>[2x]MQATKIIDGFHLVGAIDWNSR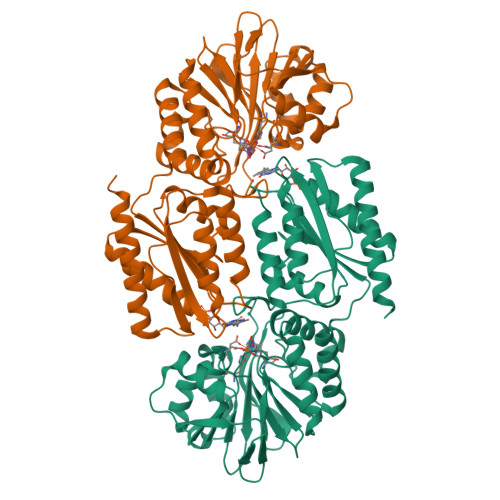DFHGYTLSPMGTTYNAYLVEDEKTTLFDTVKAEYKGELLCGIASVIDPKKIDYLVIQHLELDHAGALPALIEACQPEKIFTSSLGQKAMESHFHYKDWPVQVVKHGETLSLGKRTVTFYETRMLHWPDSMVSWFADEKVLISNDIFGQNIAASERFSDQIPVHTLERAMREYYANIVNPYAPQTLKAIETLVGAGVAPEFICPDHGVIFRGADQCTFAVQKYVEYAEQKPTNKVVIFYDSMWHSTEKMARVLAESFRDEGCTVKLMWCKACHHSQIMSEISDAGAVIVGSPTHNNGILPYVAGTLQYIKGLRPQNKIGGAFGSFGWSGESTKVLAEWLTGMGFDMPATPVKVKNVPTHADYEQLKTMAQTIARALKAKLAA>[2x]MSTKVVNVAVIGAGVVGSAFLDQLLAMKSTITYNLVLLAEAERSLISKDFSPLNVGSDWKAALAASTTKTLPLDDLIAHLKTSPKPVILVDNTSSAYIAGFYTKFVENGISIATPNKKAFSSDLATWKALFSNKPTNGFVYHEATVGAGLPIISFLREIIQ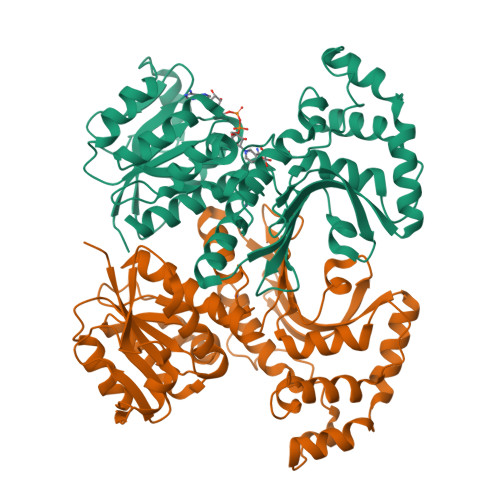TGDEVEKIEGIFSGTLSYIFNEFSTSQANDVKFSDVVKVAKKLGYTEPDPRDDLNGLDVARKVTIVGRISGVEVESPTSFPVQSLIPKPLESVKSADEFLEKLSDYDKDLTQLKKEAATENKVLRFIGKVDVATKSVSVGIEKYDYSHPFASLKGSDNVISIKTKRYTNPVVIQGAGAGAAVTAAGVLGDVIKIAQRL2,2-dimethylbutanedioic acid | C6 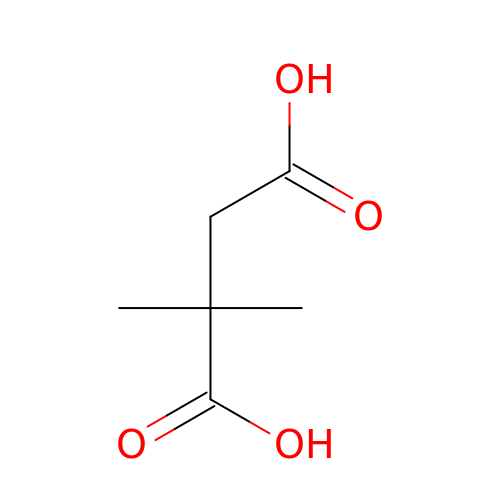H10 O4 | GOHPTLYPQCTZSE-UHFFFAOYSA-N>EEII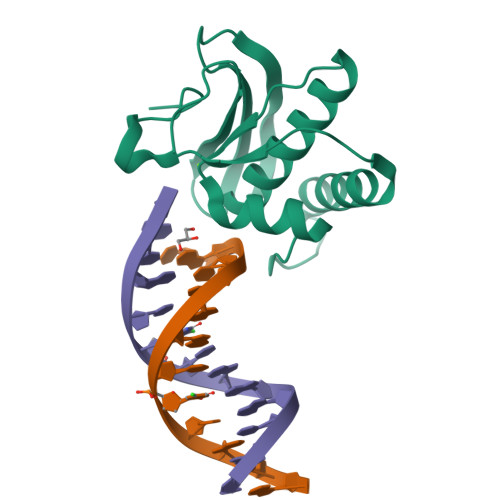WESLSVDVGSQGNPGIVEYKGVDTKTGEVLFEREPIPIGTNNMGEFLAIVHGLRYLKERNSRKPIYSNSQTAIKWVKDKKAKSTLVRNEETALIWKLVDEAEEWLNTHTYETPILKWQTDKWGEIKADYG[2x]>[4x]MTTIVSVRRNGHVVIAGDGQATLGNTVMKGNVKKVRRLYNDKVIAGFAGGTADAFTLFELFERKLEMHQGHLVKAAVELAKDWRTDRMLRKLEALLAVADETASLIITGNGDVVQPENDLIAIGSGGPYAQAAARALLENTELSAREIAEKALDIAGDICIYTNHFHTIEELSYKA;>MSE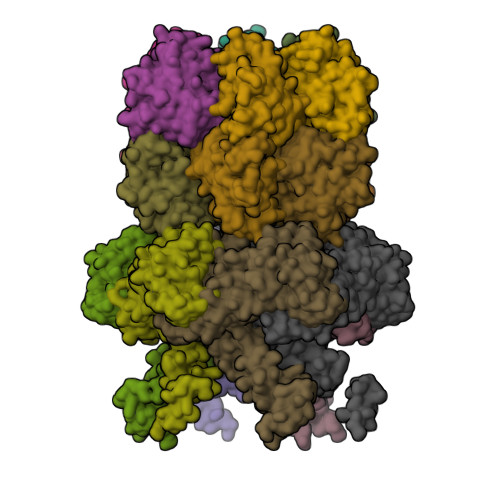MTPREIVSELDKHIIGQDNAKRSVAIALRNRWRRMQLNEELRHEVTPKNILMIGPTGVGKTEIARRLAKLANAPFIKVEATKFTEVGYVGKEVDSIIRDLTDAAVKMVRVQAIEKNRYRAEELAEERILDVLIPPAKNNWGQTEQQQEPSAARQAFRKKLREGQLDDKEIEIDLAAAPMGVEIMAPPGMEEMTSQLQSMFQNLGGQKQKARKLKIKDAMKLLIEEEAAKLVNPEELKQDAIDAVEQHGIVFIDEIDKICKRGESSGPDVSREGVQRDLLPLVEGCTVSTKHGMVKTDHILFIASGAFQIAKPSDLIPELQGRLPIRVELQALTTSDFERILTEPNASITVQYKALMATEGVNIEFTDSGIKRIAEAAWQVNESTENIGARRLHTVLERLMEEISYDASDLSGQNITIDADYVSKHLDALVADEDLSRFIL[2x]>[2x]KYRVRKNVLHLTDTEKRDFVRTVLILKEKGIYDRY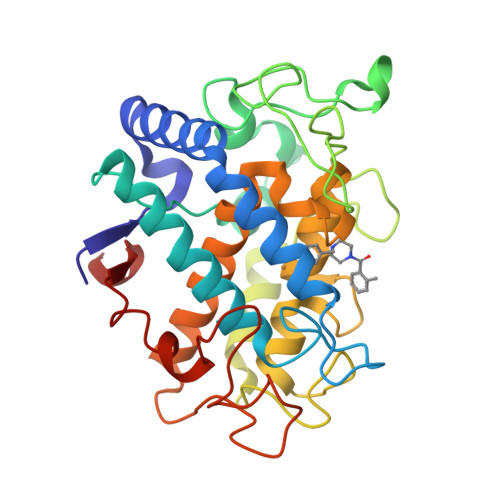IAWHGAAGKFHTPPGSDRNAAHMSSAFLPWHREYLLRFERDLQSINPEVTLPYWEWETDAQMQDPSQSQIWSADFMGGNGNPIKDFIVDTGPFAAGRWTTIDEQGNPSGGLKRNFGATKEAPTLPTRDDVLNALKITQYDTPPWDMTSQNSFRNQLEGFINGPQLHNRVHRWVGGQMGVVPTAPNDPVFFLHHANVDRIWAVWQIIHRNQNYQPMKNGPFGQNFRDPMYPWNTTPEDVMNHRKLGYVYDIELR> MQKRQSTKEEVYKDFQKQISDMNYYSCKAEVEVVGNKSPHNYVLIHTYKKTDNYKLEVISPKHLKGKSIEYQGDKILVKNPKISDVVELPNTGKNNQYLFVGDFIKNYLQNEEMKVKLSKGHLVL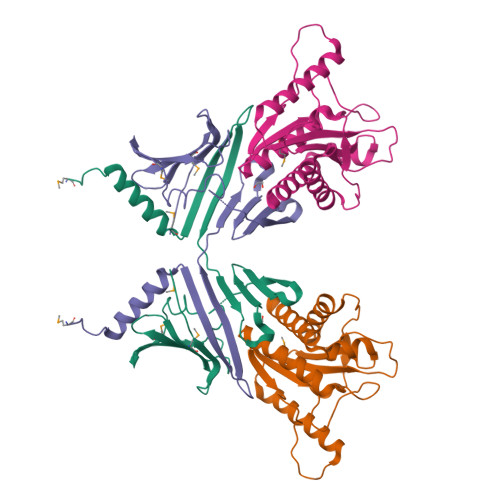ETFIPGDNKYFNKQVLYVNADTKNPEKMEVLDKEGVPRFTVKYKDFEYRN;> MKNISEDVIKYMPVTNKTIILDAGHGGIDPGALNKDKSTSEKDINLAITLKLRELIESSGGLVILTREDDSSLYKEENNKTTRQKYNENLKNRKEIISNSNANMFVSIHLNAFEQSKYYGAQTFYPKDKQDSKELSKCIQEELKRVVDKTNNREVKPRDDIYLLKDNNIPSVLIECGFLSNEKECKLLTDETYQEKIAWAIYIGIQKYLSVDKLAAA> SAFAPDFKE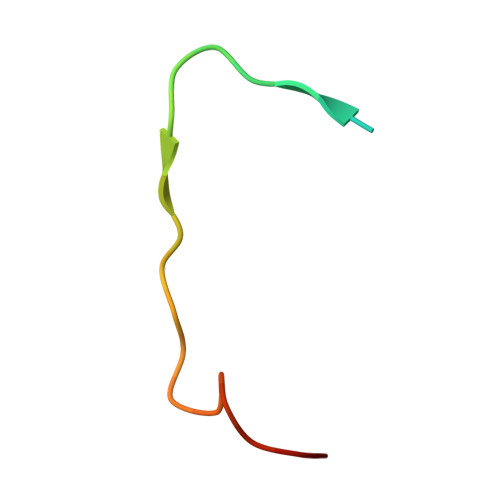LDENVEYEERESEFDIED> SSDKGKLSLQDVAELIRARACQRVVVMVGAGISTPSGIPDFRSPGSGLYSNLQQYDLPYPEAIFELPFFFHNPKPFFTLAKELYPGNYKPNVTHYFLRLLHDKGLLLRLYTQNIDGLERVSGIPASKLVEAHGTFASATCTVCQRPFPGEDIRADVMADRVPRCPVCTGVVKPDIVFFGEPLPQRFLLHVVDF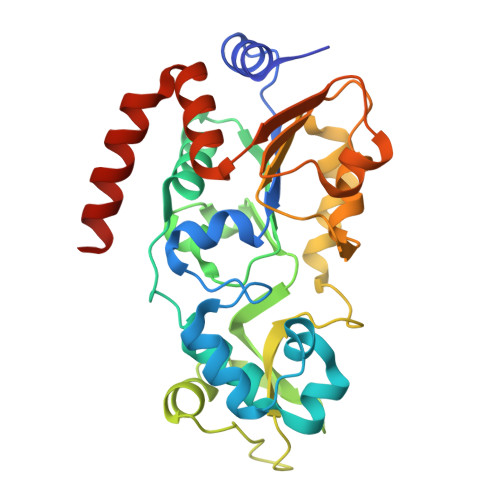PMADLLLILGTSLEVEPFASLTEAVRSSVPRLLINRDLVGPLAWHPRSRDVAQLGDVVHGVESLVELLGWTEEMRDLVQRETGKLDGPDK>[2x]QGHMAWSAQQYLKFEDERTRPARDLLAQVPLERVLNGYDLGCGPGNSTELLTDRYGVNVITGIDSDDDMLEKAADRLPNTNFGKADLATWKPAQKADLLYANAVFQWVPDHLAVLSQLMDQLE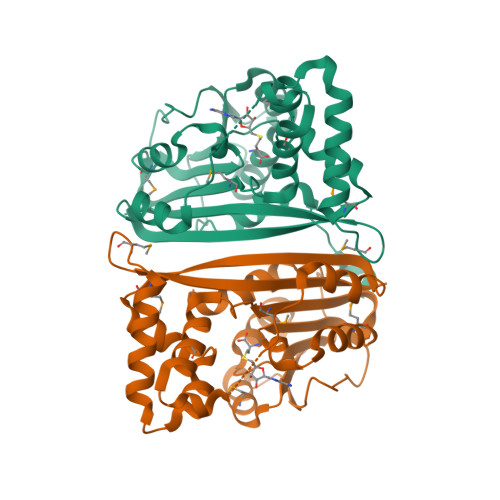SGGVLAVQMPDNLQEPTHIAMHETADGGPWKDAFSGGGLRRKPLPPPSDYFNALSPKSSRVDVWHTVYNHPMKDADSIVEWVKGTGLRPYLAAAGEENREAFLADYTRRIAAAYPPMADGRLLLRFPRLFVVAVKK2',3'-dideoxyadenosine 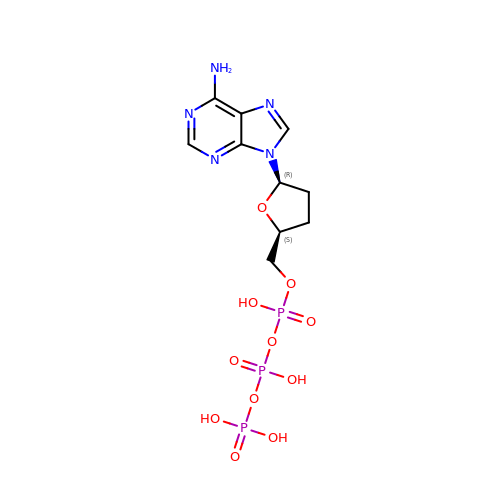triphosphate | C10 H16 N5 O11 P3 | OAKPWEUQDVLTCN-NKWVEPMBSA-N>SLVCKNALQDLSFLEHLLQVKYAP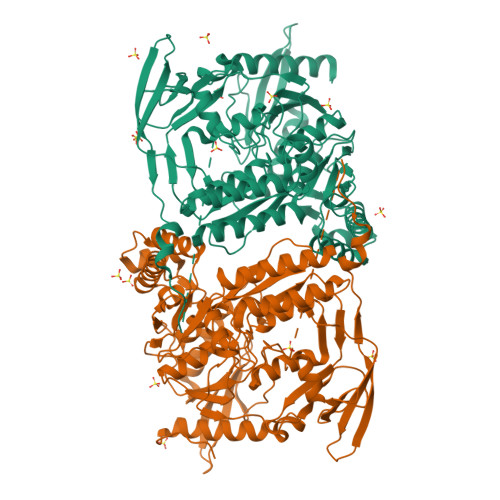KTWKEQYLGWDLVQSSVSAQQKLRTQENPSTSFCQQVLADFIGGLNDFHAGVTFFAIESAYLPYTVQKSSDGRFYFVDIMTFSSEIRVGDELLEVDGAPVQDVLATLYGSNHKGTAAEESAALRTLFSRMASLGHKVPSGRTTLKIRRPFGTTREVRVKWRYVPEGVGDLATIAPSIRAPQLQKSMRSFFPKKDDAFHRSSSLFYSPMVPHFWAELRNHYATSGLKSGYNIGSTDGFLPVIGPVIWESEGLFRAYISSVTDGDGKSHKVGFLRIPTYSWQDMEDFDPSGPPPWEEFAKIIQVFSSNTEALIIDQTNNPGGSVLYLYALLSMLTDRPLELPKHRMILTQDEVVDALDWLTLLENVDTNVESRLALGDNMEGYTVDLQVAEYLKSFGRQVLNCWSKGDIELSTPIPLFGFEKIHPHPRVQYSKPICVLINEQDFSCADFFPVVLKDNDRALIVGTRTAGAGGFVFNVQFPNRTGIKTCSLTGSLAVREHGAFIENIGVEPHIDLPFTANDIRYKGYSEYLDKVKKLVCQLINNDGTIILAEDGSFHHHHHH[2x]>[2x]MHHHHHHQIGWRREGIK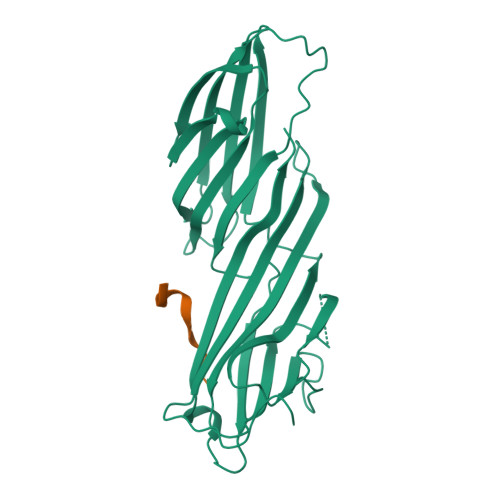YRRNELFLDVLESVNLLMSPQGQVLSAHVSGRVVMKSYLSGMPECKFGMNDKIVIEKQGKGTADETSKSGKQSIAIDDCTFHQCVRLSKFDSERSISFIPPDGEFELMRYRTTKDIILPFRVIPLVREVGRTKLEVKVVIKSNFKPSLLAQKIEVRIPTPLNTSGVQVICMKGKAKYKASENAIVWKIKRMAGMKESQISAEIELLPTNDKKKWARPPISMNFEVPFAPSGLKVRYLKVFEPKLNYSDHDVIKWVRYIGRSGIYETRC;>SDLLAWDPLFG[2x]> MNLPTAQEVQGLMARYIELVDVGDIEAIVQMFADDATVENPFGQPPIHGREQIAAFFRQGLGGGKVRACLTGPVRASHNGCGAMPFRVEMVWNGQPCALDVIDVMRFDEHGRIQTMQAYW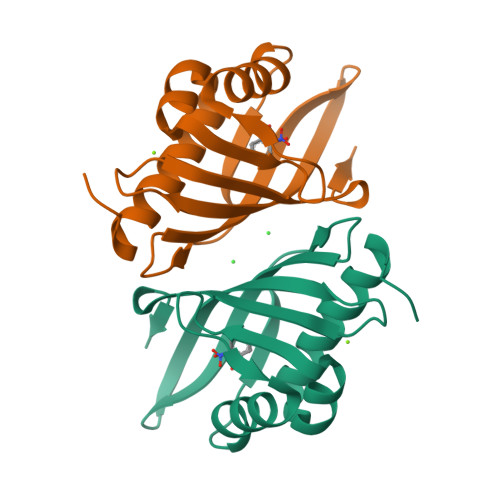SEVNLSVREPQ> GWNAYIDNLMADGTCQDAAIVGYKDSPSVW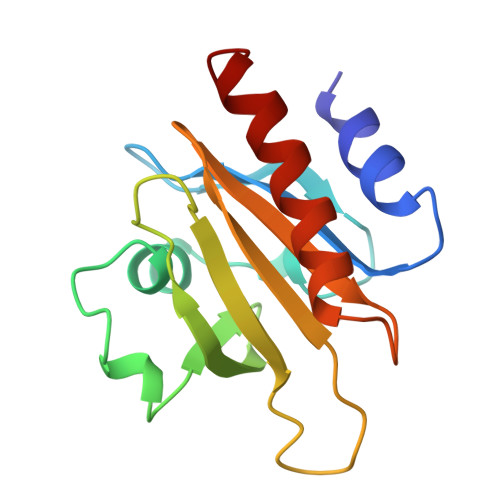AAVPGKTFVNITPAEVGVLVGKDRSSFYVNGLTLGGQKCSVIRDSLLQDGEFSMDLRTKSTGGAPTFNVTVTKTDKTLVLLMGKEGVHGGLINKKCYEMASHLRRSQY>MAAAGASRLLERLLPRHDDFARRHIGPGDKDQREMLQTLGLASIDELIEKTVPANIRLKRPLKMEDPVCENEILATLHAISSKNQIWRSYIGMGYYNCSVPQTILRNLLENSGWITQYTPYQPEVSQGRLESLLNYQTMVCDITGLDMANASLLDEGTAAAEALQLCYRHNKRRKFLVDPRCHPQTIAVVQTRAKYTGVLTELKLPCEMDFSGKDVSGVLFQYPDTEGKVEDFTELVERAHQSGSLACCATDLLALCILRPPGEFGVDIALGSSQRFGVPLGYGGPHAAFFAVRESLVRMMPGRMVGVTRDATGKEVYRLALQTREQHIRRDKATSNICTAQALLANMAAMFAIYHGSHGLEHIARRVHNATLILSEGLKRAGHQLQHDLFFDTLKIQCGCSVKEVLGRAAQRQINFRLFEDGTLGISLDETVNEKDLDDLLWIFGCESSAELVAESMGEECRGIPGSVFKRTSPFLTHQVFNSYHSETNIVRYMKKLENKDISLVHSMIPLGSCTMKLNSSSELAPITWKEFANIHPFVPLDQAQGYQQLFRELEKDLCELTGYDQVCFQPNSGAQGEYAGLATIRAYLNQKGEGHRTVCLIPKSAHGTNPASAHMAGMKIQPVEVDKYGNIDAVHLKAMVDKHKENL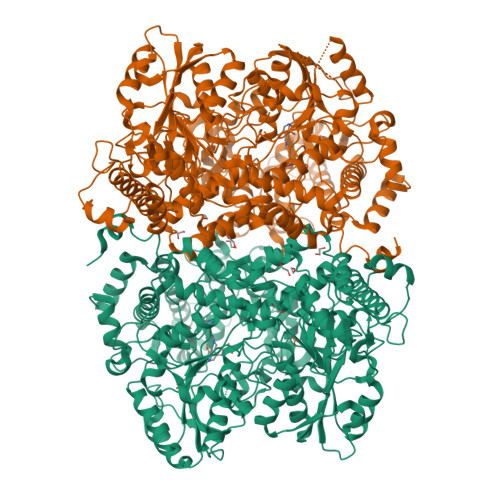AAIMITYPSTNGVFEENISDVCDLIHQHGGQVYLDGANMNAQVGICRPGDFGSDVSHLNLHKTFCIPHGGGGPGMGPIGVKKHLAPFLPNHPVISLKRNEDACPVGTVSAAPWGSSSILPISWAYIKMMGGKGLKQATETAILNANYMAKRLETHYRILFRGARGYVGHEFILDTRPFKKSANIEAVDVAKRLQDYGFHAPTMSWPVAGTLMVEPTESEDKAELDRFCDAMISIRQEIADIEEGRIDPRVNPLKMSPHSLTCVTSSHWDRPYSREVAAFPLPFVKPENKFWPTIARIDDIYGDQHLVCTCPPMEVYESPFSEQKRASSGHHHHHH[2x]> DKSIEVGRX;> GPLGSGRPSLGFTLDLHRIQRDYIDLVPKHWHVISLSLSDGGHDLCITRLQAGQAPFVLRLPLERASSRDSSVDETDVFDFHTGRAELLEIIKEI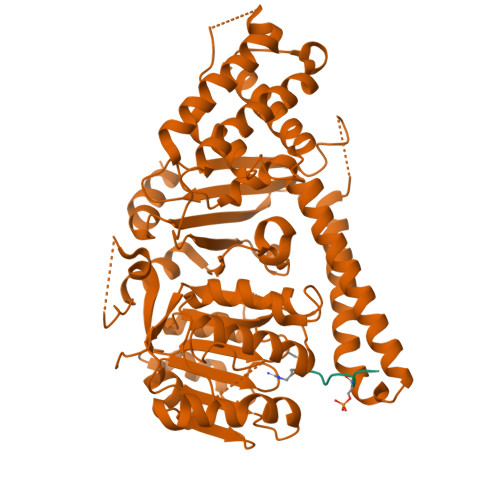NRTCHDSRDMAAKGEREKWWAEREALDQRLKELLMNIEHVWLGGFRGVFSQHGRRPELLEKFRAMFEGVLDKHLPSRRQVGRGKKGKGVAGQTKVVLDGNVLELFIGLGDATKSGADFDEELTDLLYFVVDILQFHGERNAYDEIDFDSMVVETMDALMAYHAEANAAPESDSHAHTILVLDKQLHVFPWESLPCLQGLAVSRIPSLACLRKLLLDRRRSSSQIQGEDSEEEDPRSAGHHAPLSGGTYILNPSSDLLSTQKTFESLFSTHLHSPNSWTRIISRPPTEPEFLSALTHSPILLYFGHGSGAQYIRSRNIRHLDHCRATVLLMGCSSAALTAKGEFEPSGPVWNYMLAGAPAVVGTLWDVTDRDIDRFAGGVLEGWGVLPEGCMGEKNGKKKAGRNGLSLVQAVAKARDRCRFRYVTAAAAVVYGIPVYVDVDGKSKD Protein fem‐1 homolog B (FEM1B) is a substrate recognition protein of the Cullin‐RING (CUL2) E3 ligase and plays a critical role in regulating proteins in the cell (Chen et al., 2021, 2024; Hughes et al., 2021; Kramer & Zhang, 2022; Manford et al., 2021; Raiff et al., 2025; Zhao et al., 2021). FEM1B plays a crucial role in balancing the reductive stress response in the cell by degrading key proteins involved in redox sensing and management (Manford et al., 2021). FEM1B binds multiple degron substrates with distinct recognition sequences, which suggests FEM1B has multiple recognition sites for substrate binding. Here, we describe the development of a stable construct of FEM1B, the results of a protein‐observed NMR‐based fragment screen using this construct, and the X‐ray structures of some of the fragment hits when bound to the protein.

The X‐ray structures were determined for six additional molecules (VU0412674, VU0417412, VU0421763, VU0023775, VU0081201, and VU0432623) in complex with FEM1B. The six additional molecules which are classified as chemical shift pattern 3 sit in the same binding pocket. The other six fragments bound to the same site in the FEM1B substrate binding pocket, a region typically important for identifying C‐terminal prolines of degron substrates in a non‐covalent manner. VU0421763 (KD = 0.34 mM) does not sit in the same closed position, but Phe130 forms a hydrophobic interaction with the pyrazolo pyrimidine ring of the molecule, while Tyr84 sits in a flipped orientation compared to its position with VU0412674 or VU0417412 present.

>[2x]GHMEGLAGYVYKAASEGKVLTLAALLLNRSESDIRYLLGYVSQQGGQRSTPLIIAARNGHAKVVRLLLEHYRVQTQQTGTVRFDGYVIDGATALWCAAGAGHFEVVKLLVSHGANVNHTTVTNSTPLRAACFDGRLDIVKYLVENNANISIANKYDNTCLMIAAYKGHTDVVRYLLEQRADPNAKAHCGATALHFAAEAGHIDIVKELIKWRAAIVVNGHGMTPLKVAAESCKADVVELLLSHADCDRRSRIEALELLGASFANDRENYDIIKTYHYLYLAMLERFQDGDNILEKEVLPPIHAYGNRTECRNPQELESIRQDRDALHMEGLIVRERILGGGGSGGGSKKRLLLGLDR> VELTESTRTIPLDEAGGTTTLTARQFT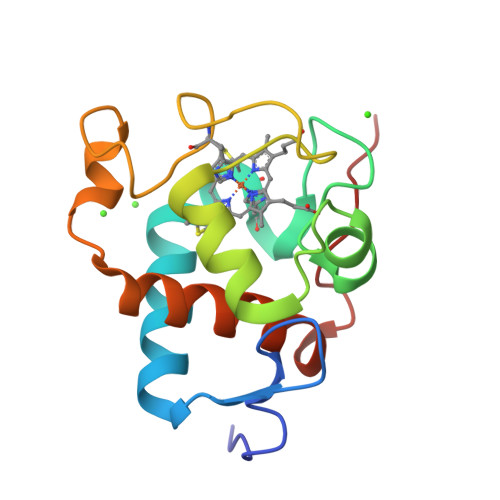NGQKIFVDTCTQCHLQGKTKTNNNVSLGLADLAGAEPRRDNVLALVEFLKNPKSYDGEDDYSELHPNISRPDIYPEMRNYTEDDIFDVAGYTLIAPKLDERWGGTIYF>MDFFSLAEELPQNEDLLESEDDAPIIKLINAMLGEAIKEGASDIHIETFEKTLSIRFRVDGVLREVLAPSRKLSSLLVSRVKVMAKLDIAEKRVPQDGRISLRIGGRAVDVRVSTMPSSHGERVVMRLLDKNATRLDLHSLGMTAHNHDNFRRLIKRPHGIILVTGPTGSGKSTTLYAGLQELNSSERNILTVEDPIEFDIDGIGQTQVNPRVDMTFARGLRAILRQDPDVVMVGEIRDLETAQIAVQASLTGHLVMSTLHTNTAVGAVTRLRDMGIEPFLISSSLLGVLAQRLVRTLCPDCKEPYEADKEQRKLFDSKKKEPLILYRATGCPKCNHKGYRGRTGIHELLLVDDALQELIHSEAGEQAMEKHIRATTPSIRDDGLDKVRQGITSLEEVMRVTKESGSGSGSGAVDMFIKIGDVKGESKDKTHAEEIDVLAWSWGMSQSGSMHMGGGGGAGKVNVQDLSFTKYIDKSTPNLMMACSSGKHYPQAKLTIRKAGGENQVEYLIITLKEVLVSSVSTGGSGGEDRLTENVTLNFAQVQVDYQPQKADGAKD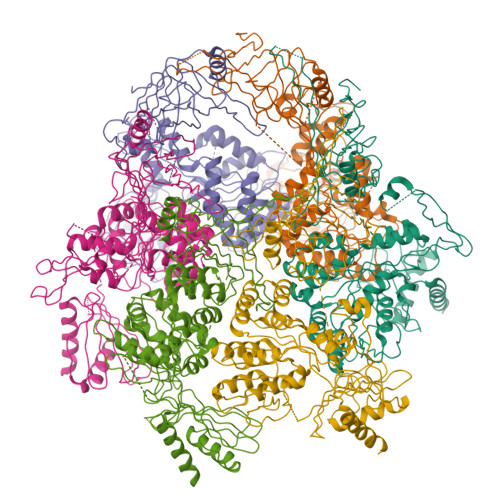GGPVKYGWNIRQNVQALEHHHHHH[6x]> GGGYPYFIPKGK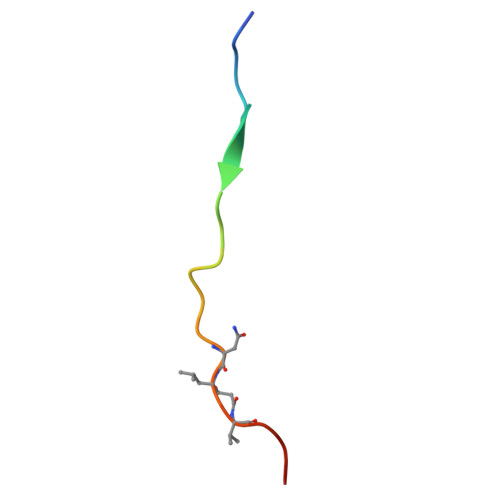GEVNXVAEPX> MTLEKFVDALPIPDTLKPVQQSKEKTYYEVTMEECTHQLHRDLPPTRLWGYNGLFPGPTIEVKRNENVYVKWMNNLPSTHFLPIDHTIHHSDSQHEEPEVKTVVHLHGGVTPDDSEGYPEAWFSKDFEQTGPYFKREVYHYPNQQRGAILWYHDHAMALTRLNVYAGLVGAYIIHDPKEKRLKLPS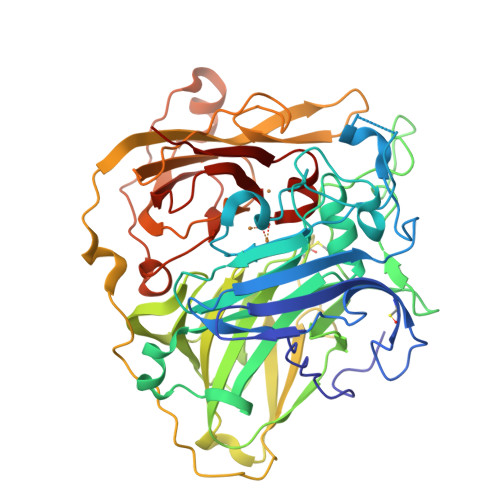DEYDVPLLITDRTINEDGSLFYPSAPENPSPSLPNPSIVPAFCGETILVNGKVWPYLEVEPRKYRFRVINASNTRTYNLSLDNGGDFIQIGSDGGLLPRSVKLNSFSLAPAERYDIIIDFTAYEGESIILANSAGCGGDVNPETDANIMQFRVTKPLAQKDESRKPKYLASYPSVQHERIQNIRTLKLAGTQDEYGRPVLLLNNKRWHDPVTETPKVGTTEIWSIINPTRGTHPIHLHLVSFRVLDRRPFDIARYQESGELSYTGPAVPPPPSEKGWKDTIQAHAGEVLRIAATFGPYSGRYVWHCHILEHEDYDMMRPMDITDPHK The majority of traits controlled by rhl transcription factor RhlR depend on PqsE, a dispensable thioesterase in Pseudomonas Quinolone Signal (PQS) biosynthesis that interferes with RhlR through an enigmatic mechanism likely involving direct interaction of both proteins. Here we show that PqsE and RhlR form a 2:2 protein complex that, together with RhlR agonist N-butanoyl-L-homoserine lactone (C4-HSL), solubilizes RhlR and thereby renders the otherwise insoluble transcription factor active. PqsE is a thioesterase that triggers transcription of the RhlR regulon through a hitherto cryptic mechanism, which we identify here as involving a significant chaperone-like component that enhances the stability of RhlR via protein complex formation. In common with many other gram-negative bacteria, two QS circuits use N-acyl-L-homoserine lactones (HSLs) as autoinducers, namely N-(3-oxododecanoyl)-L-HSL (3-oxo-C12-HSL) and N-butanoyl-L-HSL (C4-HSL), which are produced by autoinducer synthases LasI and RhlI and activate the LuxR-type transcription factors LasR and RhlR, respectively.

Recombinant production of the fusion protein was straightforward but required C4-HSL or mBTL, reflecting the stability-enhancing effect of these ligands. The fusion protein in the presence of mBTL crystallized in space group I422 with one homodimer in the asymmetric unit, but the linker between PqsE and RhlR was flexible and did not yield visible electron density, whereas mBTL was found in the ligand binding domain (LBD) of RhlR. The PqsE segment adopted the same dimeric configuration as in the free protein but with a slightly twisted arrangement. The RhlR sequence displayed the expected homodimeric structure of a LuxR-type transcription factor and C4-HSL as well as mBTL were found in the anticipated ligand binding site (Supplementary Fig. 4a/b).

>MGHHHHHHAENLYFQGHMLRLSAPGQLDDDLCLLGDVQVPVFLLRLGEASWALVEGGISRDAELVWADLCRWVADPSQVHYWLITHKHYDHCGLLPYLCPRLPNVQVLASERTCQAWKSESAVRVVERLNRQLLRAEQRLPEACAWDALPVRAVADGEWLELGPRHRLQVIEAHGHSDDHVVFYDVRRRRLFCGDALGEFDEAEGVWRPLVFDDMEAYLESLERLQRLPTLLQLIPGHGGLLRGRLAADGAESAYTECLRLCRRLLWRQSMGESLDELSEELHRAWGGQSVDFLPGELHLGSMRRMLEILSRQALPLDSGSETPGTSESATPESGPGTMRNDGGFLLWWDGLRSEMQPIHDSQGVFAVLEKEVRRLGFDYYAYGVRHTIPFTRPKTEVHGTYPKAWLERYQMQNYGAVDPAILNGLRSSEMVVWSDSLFDQSRMLWNEARDWGLCVGATLPIRAPNNLLSVLSVARDQQNISSFEREEIRLRLRCMIELLTQKLTDLEHPMLMSNPVCLSHREREILQWTADGKSSGEIAIILSISESTVNFHHKNIQKKFDAPNKTLAAAYAAALGLI[2x]> MLEQPYLDLAKKVLDEGHFKPDRTHTGTYSIFGHQMRFDLSKGFPLLTTKKVPFGLIKSELLWFLHGDTNIRFLLQHRNHIWDEWAFEKWVKSDEYHGPDMTDFGHRSQKDPEFAAVYHEEMAKFDDRVLHDDAFAAKYGDLGLVYGSQWRAWHTSKGDTIDQLGDVIEQIKTHPYSRRLIVSAWNPEDVPTMALPPCHTLYQFYVNDGKLSLQLYQRSADIFLGVPFIIASYALLTHLVAHECGLEVGEFIHTFGDAHLYVNHLDQIKEQLSRTPRPAPTLQLNPDKHDIF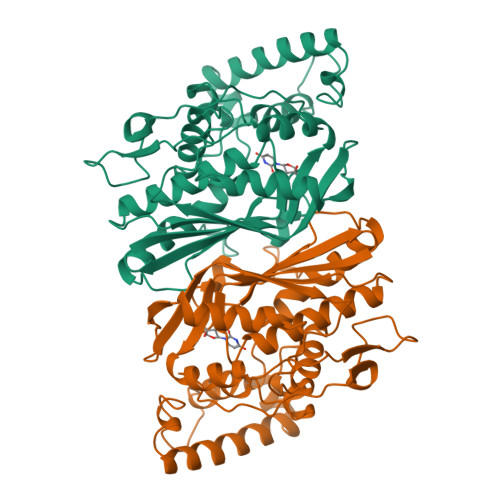DFDMKDIKLLNYDPYPAIKAPVAV> MAEKIELSKRDRLRVA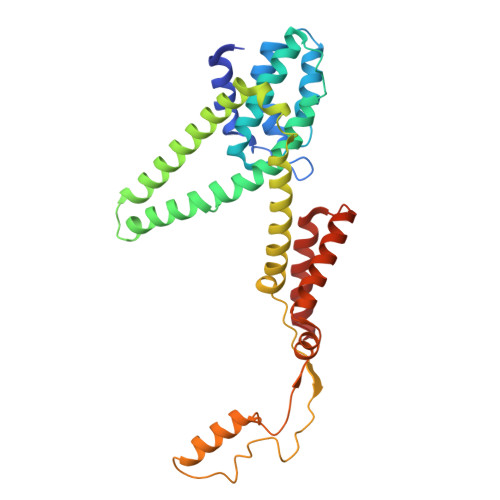WRSTFIQGSWNYERMQNGGWAFSMIPAIKKLYKTKEDRSSALKRHLEFFNTHPYIASPILGVTLALEEERANGAEVDDVAIQGVKVGMMGPLAGVGDPVFWFTIRPMLGALGASLALSGNILGPILFFVAWNVIRWGFMWYTQEFGYKAGSKITDDLSGGLLQDITKGASILGMFVLAALVQRWVNIQFAPIISKVKLDEGAYIDWSHLPQGAQGIKTALQQQQAGLALSEIKVTTLQNNLDNLIPGLAAVALTFLCMWLLKKKISPIIIILGLFVVGIVGHLIGLL>MPRGSRSAASRPASRPAAPSAHPPAHPPPSAAAPAPAPSGQPGLMAQMATTAAGVAVGSAVGHVMGSALTGAFSGGSSEPSQPAVQQAPTPAAPQPLQ[18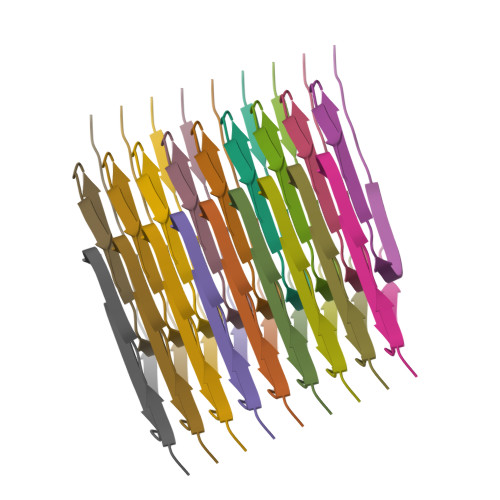x]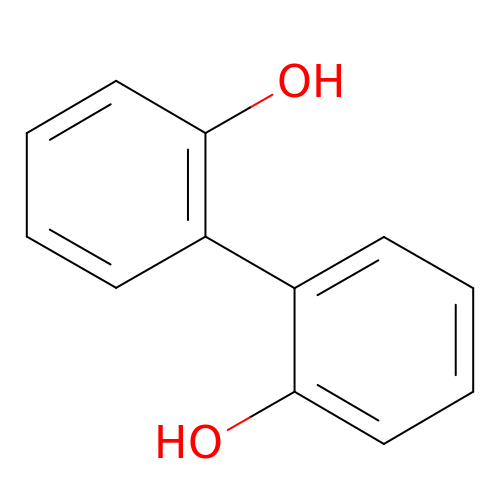2-(2-hydroxyphenyl)phenol | C12 H10 O2 | IMHDGJOMLMDPJN-UHFFFAOYSA-N>MVLYFIGLGLMDERDITVKGLEIAKKCDYVFAEFYTSLMAGTTLGRIQKLIGKEIRVLSREDVELNFENIVLPLAKENDVAFLTPGDPLVATTHAELRIRAKRAGVESYVIHAPSIYSAVGITGLHIYKFGKSATVAYPEGNWFPTSYYDVIKENAERGLHTLLFLDIKAEKRMYMTANEAMELLLKVEDM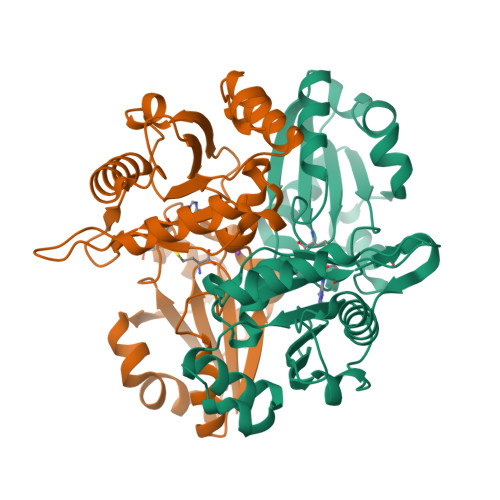KKGGVFTDDTLVVVLARAGSLNPTIRAGYVKDLIREDFGDPPHILIVPGKLHIVEAEYLVEIAGAPREILRVNV[2x]One enzyme in particular, 2-aminomuconate-6-semialdehyde dehydrogenase (AMSDH), is responsible for oxidizing the unstable metabolic intermediate 2-aminomuconate-6-semialdehyde (2-AMS) to 2-aminomuconate (2-AM). On the basis of sequence alignment, AMSDH is a member of the hydroxymuconic-semialdehyde dehydrogenase (HMSDH) family under the aldehyde dehydrogenase (ALDH) superfamily. The complete AMSDH model includes four polypeptides per asymmetric unit describing one homotetramer. Each monomer of AMSDH contains three domains: a subunit interaction domain, a catalytic domain and an NAD+ binding domain.

To probe the function of Glu268, we constructed an alanine mutant and found that it exhibited no detectable activity in steady-state kinetic assays. We determined the crystal structure of E268A co-crystallized with NAD+ and refined it to 2.00 Å resolution. The overall structure aligns very well with the wild-type binary complex structure with an r.m.s.d. of 0.139 Å. The active site of E268A also resembles the native AMSDH structure. Interestingly, E268A exhibits completely different pre-steady state activity than the wild-type enzyme.

>[4x]SQLLNYIDGNFVTSASSFANINPVNGKLISDVFEADAKQVNEAVVAAQNALKGPWGKLSVQDRAALIHKIADGIQARFEEFVAAEVADTGRPVHQARTLDIPRAIANFRTFADLAKTSHTDLFEMSTSDGSGALNYTVRKPLGVIGVISPWNLPLLLFTWKVAPALACGNTVVAKPSEESPSSATLLAEVMHDAGVPPGVFNLIHGFGKDSAGEFLTQHPGISALTFTGESKTGSTIMKAVADGVKEVSFALGGKNAAVVFADADLDAAIEGVLRSSFTNSGQVCLCSERVYVHRSIFDEFVSGLKVEAERLVVGYPDQDGVNMGPLISHGHRDKVLSYYRLAVDEGATVVTGGGVPKFNDERDQGAYVQPTIWTGLSDKARCVTEEIFGPVCHISPFDDEDEVINRVNDSNYGLACAIWTTNLSRAHRVSRQIHVGLVWVNTWYLRDLRTPFGGVKLSGLGREGGRFSMDFYSDIANICIKI Growth/differentiation factors 8 and 11 (GDF8/myostatin and GDF11/BMP11, respectively) are two closely related members of the activin/inhibin subclass that share ~90% sequence identity in their mature, C-terminal signaling domains and ~52% identity in their N-terminal prodomains. Similar to other TGFβ ligands, GDF8 and GDF11 are disulfide-linked dimers that are initially synthesized as precursors, which are cleaved by furin-like proteases to separate the N-terminal prodomain from the C-terminal mature domain. The ligand dimer elicits signal transduction by symmetrically binding two type II and two type I transmembrane serine/threonine kinase receptors. Similar to other ligands in the activin/inhibin subclass, GDF8 and GDF11 predominantly signal through the type II receptors, activin receptor kinase IIA (ActRIIA; ACVR2A) and ActRIIB (ACVR2B) and the type I receptors, activin-like receptor kinase 4 (ALK4; ACVR1B) and ALK5 (TβRI).

The complex of the GDF11 dimer bound to two molecules of FS288 was resolved using X-ray crystallography to 2.35 Å. This is the first structure of GDF11 bound to a known antagonist. Similar to previous ligand:follistatin structures, two molecules of FS288 bind symmetrically to wrap around the GDF11 dimer occluding both type II and type I receptor binding sites. As expected, follistatin domains 1 (D1) and D2 overlap with the type II binding epitope, whereas the follistatin N-terminal domain (ND) occupies the type I binding slot. The overall structure of GDF11:FS288 is highly similar to that of the GDF8:FS288 complex (Fig. 3a; overall root-mean-square deviation (RMSD) = 0.657 Å). Nonetheless, the structure of GDF11:FS288 reveals minor changes in the positioning of residues in the helix of ND. For example, F47 of FS288 is pushed inward to accommodate the larger side chain of M50 in GDF11 versus V50 in GDF8. This is consistent with other ligand:FS structures, showing that the ND helix is quite plastic in its “molding” to accommodate ligand differences at the type I interface. However, examination of the type I interface revealed two unique interactions in the wrist of GDF11 compared to GDF8. The second unique feature of GDF11 is the formation of an additional hydrogen bond between the backbone (Y49A) of the pre-helix loop and Q62A located on the C-terminal side of the wrist helix.

>[2x]NLGLDCDEHSSESRCCRYPLTVDFEAFGWDWIIAPKRYKANYCSGQCEYMFMQKYPHTHLVQQANPRGSAGPCCTPTKMSPINMLYFNDKQQIIYGKIPGMVVDRCGCS;>GNCWLRQAKNGRCQVLYKTELSKEECCSTGRLSTSWTEEDVNDNTLFKWMIFNGGAPNCIPCKETCENVDCGPGKKCRMNKKNKPRCVCAPDCSNITWKGPVCGLDGKTYRNECALLKARCKEQPELEVQYQGRCKKTCRDVFCPGSSTCVVDQTNNAYCVTCNRICPEPASSEQYLCGNDGVTYSSACHLRKATCLLGRSIGLAYEGKCIKAKSCEDIQCTGGKKCLWDFKVGRGRCSLCDELCPDSKSDEPVCASDNATYASECAMKEAACSSGVLLEVKHSGSCN[2x]>MIAHLINTDIGNRGVLKVYLDYRRKNFNFLHNSTKMFLDNLERVLIVTGFPIPPMMVAETDGPPGALAIYRAVEMLGGKAEILTYSEVEKALEPFGVSLARTPEPEDYSLIISVETPGRAADGRYYSMSALEIKRDPLDGIFLKARALGIPTIGVGDGGNEIGMGKIRELVVGHVPHGEKIASVVETDELIVSAVSNWGAYGLVAQASIEVGRNLLEGWDERRVIEAISSAGLIDGVSKTLAPSVD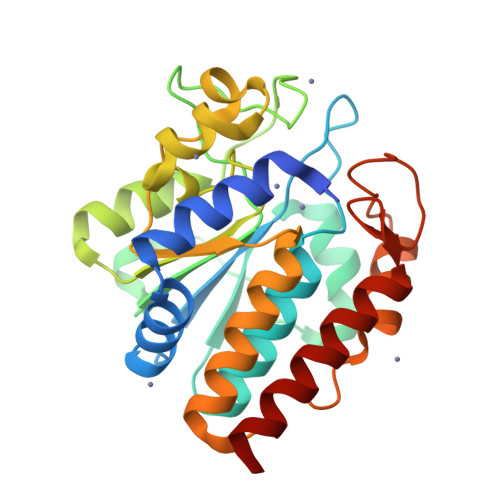GIRLMVHEGIVELLKAVVDEAIKL[6x]> MSLTEQIEQFASRFRDDDATLQSRYSTLSELYDIMELLNSPEDYHFFLQAVIPLLLNQLKEVPISYDAHSPEQKLRNSMLDIFNRCLMNQTFQPYAMEVLEFLLSVLPKENEENGILCMKVLTTLFKSFKSILQDKLDSFIRIIIQIYKNTPNLINQTFYEAGKAEQGDLDSPKEPQADELLDEFSKNDEEKDFPSKQSSTEPRFENSTSSNGLRSSMFSFKILSECPITMVTLYSSYKQLTSTSLPEFTPLIMNLLNIQIKQQQEAREQAESRGEHFTSISTEIINRPAYCDFILAQIKATSFLAYVFIRGYAPEFLQDYVNFVPDLIIRLLQDCPSELSSARKELLHATRHILSTNYKKLFLPKLDYLFDERILIGNGFTMHETLRPLAYSTVADFIHNIRSELQLSEIEKTIKIYTGYLLDESLALTVQIMSAKLLLNLVERILKLGKENPQEAPRAKKLLMIIIDSYMNRFKTLNRQYDTIMKYYGRYETHKKEKAEKLKNSIQDNDKESEEFMRKVLEPSDDDHLMPQPKKEDINDSPDVEMTESDKVVKNDVEMFDIKNYAPILLLPTPTNDPIKDAFYLYRTLMSFLKTIIHDLKVFNPPPNEYTVANPKLWASVSRVFSYEEVIVFKDLFHECIIGLKFFKDHNEKLSPETTKKHFDISMPSLPVSATKDARELMDYLAFMFMQMDNATFNEIIEQELPFVYERMLEDSGLLHVAQSFLTSEITSPNFAGILLRFLKGKLKDLGNVDFNTSNVLIRLFKLSFMSVNLFPNINEVVLLPHLNDLILNSLKYSTTAEEPLVYFYLIRTLFRSIGGGRFENLYRSIKPILQVLLQSLNQMILTARLPHERELYVELCITVPVRLSVLAPYLPFLMKPLVFALQQYPDLVSQGLRTLELCIDNLTAEYFDPIIEPVIDDVSKALFNLLQPQPFNHAISHNVVRILGKLGGRNRQFLKPPTDLTEKTELDIDAIADFKINGMPEDVPLSVTPGIQSALNILQSYKSDIHYRKSAYKYLTCVLLLMTKSSAEFPTNYTELLKTAVNSIKLERIGIEKNFDLEPTVNKRDYSNQENLFLRLLESVFYATSIKELKDDAMDLLNNLLDHFCLLQVNTTLLNKRNYNGTFNIDLKNPNFMLDSSLILDAIPFALSYYIPEVREVGVLAYKRIYEKSCLIYGEELALSHSFIPELAKQFIHLCYDETYYNKRGGVLGIKVLIDNVKSSSVFLKKYQYNLANGLLFVLKDTQSEAPSAITDSAEKLLIDLLSITFADVKEEDLGNKVLENTLTDIVCELSNANPKVRNACQKSLHTISNLTGIPIVKLMDHSKQFLLSPIFAKPLRALPFTMQIGNVDAITFCLSLPNTFLTFNEELFRLLQESIVLADAEDESLSTNIQKTTEYSTSEQLVQLRIACIKLLAIALKNEEFATAQQGNIRIRILAVFFKTMLKTSPEIINTTYEALKGSLAENSKLPKELLQNGLKPLLMNLSDHQKLTVPGLDALSKLLELLIAYFKVEIGRKLLDHLTAWCRVEVLDTLFGQDLAEQMPTKIIVSIINIFHLLPPQADMFLNDLLLKVMLLERKLRLQLDSPFRTPLARYLNRFHNPVTEYFKKNMTLRQLVLFMCNIVQRPEAKELAEDFEKELDNFYDFYISNIPKNQVRVVSFFTNMVDLFNTMVITNGDEWLKKKGNMILKLKDMLNLTLKTIKENSFYIDHLQLNQSIAKFQALYLRFTELSERDQNPLLLDFIDFSFSNGIKASYSLKKFIFHNIIASSNKEKQNNFINDATLFVLSDKCLDARIFVLKNVINSTLIYEVATSGSLKSYLVEDKKPKWLELLHNKIWKNSNAILAYDVLDHHDLFRFELLQLSAIFIKADPEIIAEIKKDIIKFCWNFIKLEDTLIKQSAYLVTSYFISKFDFPIKVVTQVFVALLRSSHVEARYLVKQSLDVLTPVLHERMNAAGTPDTWINWVKRVMVENSSSQNNILYQFLISHPDLFFNSRDLFISNIIHHMNKITFMSNSNSDSHTLAIDLASLILYWENKTLEITNVNNTKTDSDGDVVMSDSKSDINPVEADTTAIIVDANNNSPISLHLREACTAFLIRYVCASNHRAIETELGLRAINILSELISDKHWTNVNVKLVYFEKFLIFQDLDSENILYYCMNALDVLYVFFKNKTKEWIMENLPTIQNLLEKCIKSDHHDVQEALQKVLQVIMKAIKAQGVSVIIEEESPGKTFIQMLTSVITQDLQETSSVTAGVTLAWVLFMNFPDNIVPLLTPLMKTFSKLCKDHLSISQPKDAMALEEARITTKLLEKVLYILSLKVSLLGDSRRPFLSTVALLIDHSMDQNFLRKIVNMSRSWIFNTEIFPTVKEKAAILTKMLAFEIRGEPSLSKLFYEIVLKLFDQEHFNNTEITVRMEQPFLVGTRVEDIGIRKRFMTILDNSLERDIKERLYYVIRDQNWEFIADYPWLNQALQLLYGSFNREKELSLKNIYCLSPPSILQEYLPENAEMVTEVNDLELSNFVKGHIASMQGLCRIISSDFIDSLIEIFYQDPKAIHRAWVTLFPQVYKSIPKNEKYGFVRSIITLLSKPYHTRQISSRTNVINMLLDSISKIESLELPPHLVKYLAISYNAWYQSINILESIQSNTSIDNTKIIEANEDALLELYVNLQEEDMFYGLWRRRAKYTETNIGLSYEQIGLWDKAQQLYEVAQVKARSGALPYSQSEYALWEDNWIQCAEKLQHWDVLTELAKHEGFTDLLLECGWRVADWNSDRDALEQSVKSVMDVPTPRRQMFKTFLALQNFAESRKGDQEVRKLCDEGIQLSLIKWVSLPIRYTPAHKWLLHGFQQYMEFLEATQIYANLHTTTVQNLDSKAQEIKRILQAWRDRLPNTWDDVNMWNDLVTWRQHAFQVINNAYLPLIPALQQSNSNSNINTHAYRGYHEIAWVINRFAHVARKHNMPDVCISQLARIYTLPNIEIQEAFLKLREQAKCHYQNMNELTTGLDVISNTNLVYFGTVQKAEFFTLKGMFLSKLRAYEEANQAFATAVQIDLNLAKAWAQWGFFNDRRLSEEPNNISFASNAISCYLQAAGLYKNSKIRELLCRILWLISIDDASGMLTNAFDSFRGEIPVWYWITFIPQLLTSLSHKEANMVRHILIRIAKSYPQALHFQLRTTKEDFAVIQRQTMAVMGDKPDTNDRNGRRQPWEYLQELNNILKTAYPLLALSLESLVAQINDRFKSTTDEDLFRLINVLLIDGTLNYNRLPFPRKNPKLPENTEKNLVKFSTTLLAPYIRPKFNADFIDNKPDYETYIKRLRYWRRRLENKLDRASKKENLEVLCPHLSNFHHQKFEDIEIPGQYLLNKDNNVHFIKIARFLPTVDFVRGTHSSYRRLMIRGHDGSVHSFAVQYPAVRHSRREERMFQLYRLFNKSLSKNVETRRRSIQFNLPIAIPLSPQVRIMNDSVSFTTLHEIHNEFCKKKGFDPDDIQDFMADKLNAAHDDALPAPDMTILKVEIFNSIQTMFVPSNVLKDHFTSLFTQFEDFWLFRKQFASQYSSFVFMSYMMMINNRTPHKIHVDKTSGNVFTLEMLPSRFPYERVKPLLKNHDLSLPPDSPIFHNNEPVPFRLTPNIQSLIGDSALEGIFAVNLFTISRALIEPDNELNTYLALFIRDEIISWFSNLHRPIIENPQLREMVQTNVDLIIRKVAQLGHLNSTPTVTTQFILDCIGSAVSPRNLARTDVNFMPWF

In Saccharomyces cerevisiae, the 1.8-MDa coactivator SAGA (Spt–Ada–Gcn5–acetyltransferase) complex1 was reported to be required for genome-wide transcription by RNA Pol II, and proposed to function as a general cofactor. Yeast SAGA is composed of 19 subunits, which are categorized into four modules, namely HAT (Gcn5, Ada2, Ada3, and Sgf29), DUB (Ubp8, Sgf11, Sgf73, and Sus1), TAF (Taf5, Taf6, Taf9, Taf10, and Taf12), and SPT (Tra1, Ada1, Spt3, Spt7, Spt8, and Spt20). The largest SAGA component Tra1 (3744 residues) in the SPT module was shown to directly interact with the acidic activation domain of TFs, such as VP16, GCN4, Gal4, and HAP44, which help recruit SAGA to promoter regions of target genes. SAGA and NuA4 are two major acetyltransferases in yeast and share the largest subunit Tra1.

We successfully purified an endogenous SAGA complex that contains all 19 subunits from fermented S. cerevisiae cells after optimization of growth conditions. The structure of SAGA was determined by single-particle cryo-EM analysis at a resolution up to 6.9 Å. The overall shape of SAGA resembles an open padlock, and can be divided into lobes A and B. Finally, the cryo-EM map of lobe A was reconstructed at 4.6 Å at FSC = 0.143. Tra1 is composed of HEAT (Finger, N-clasp, Ring, and C-clasp), FAT, FRB, PI3K/PI4K, and FATC domains from the N- to the C-terminus. We eventually generated an alanine-substituted structure of Tra1 consisting of alanine, glycine, and proline residues. Tra1 is characteristic of a helical solenoid fold and arranged into a “θ”-like structure, in which a Ring motif (1140–2442) within the HEAT domain forms the ring. Tra1 functions as a base to organize other subunits in lobe B of SAGA. Structural comparison of free Tra1 with its complex state revealed only regional conformational adjustments upon SAGA assembly, which reflects the structural rigidity of the solenoid fold of Tra1. In addition, the elongated ridge surface formed by FAT, PI3K/PI4K, C-Clasp, and Ring-C of Tra1 constitutes the major contact interface with lobe B.> DRVYIHPFHLVIHNESTCEQLAKANAGKPKDPTFIPAPIQAKTSPVDEKALQDQLVLVAAKLDTEDKLRAAMVGMLANFLGFRIYGMHSELWGVVHGATVLSPTAVFGTLASLYLGALDHTADRLQAILGVPWKDKQCTSRLDAHKVLSALQAVQGLLVAQGRADSQAQLLLSTVVGVFTAPGLHLKQPFVQGLALYTPVVLPRSLDFTELDVAAEKIDRFMQAVTGWKTGSSLMGASVDSTLAFNTYVHFQGKMKGFSLLAEPQEFWVDQSTSVSVPMLSGMGTFQHWSDIQDQFSVTQVPFTESASLLLIQPHYASDLDKVEGLTFQQNSLNWMKKLSPRTI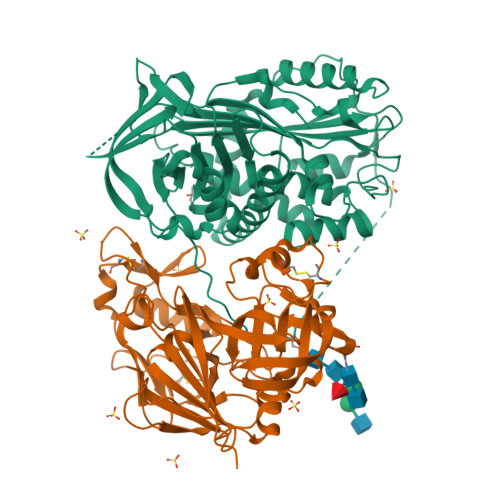HLTMPQLVLQGSYDLQDLLAQAELPAILHTELNLQKLSNDRIRVGEVLNSIFFELEADEREPTESTQQLNKPEVLEVTLNRPFLFAVYDQSATALHFLGRVANPLSTAHHHHHH;> LTLGNTTSSVILTNYMDTQYYGEIGIGTPPQTFKVVFDTGSSNVWVPSSKCSRLYTACVYHKLFDASDSSSYKHNGTELTLRYSTGTVSGFLSQDIITVGGITVTQMFGEVTEMPALPFMLAEFDGVVGMGFIEQAIGRVTPIFDNIISQGVLKEDVFSFYYNRDSENSQSLGGQIVLGGSDPQHYEGNFHYINLIKTGVWQIQMKGVSVGSSTLLCEDGCLALVATGASYISGSTSSIEKLMEALGAKKRLFDYVVKCNEGPTLPDISFHLGGKEYTLTSADYVFQESYSSKKLCTLAIHAMDIPPPTGPTWALGATFIRKFYTEFDRRNNRIGFALAR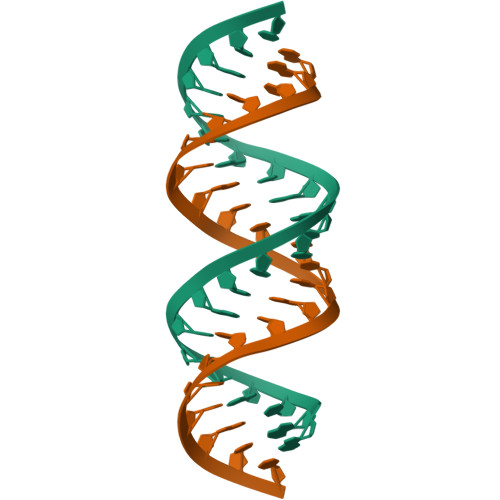>[2x]GGUAGACGCUUCGGCGUUUGCC> GEMNVDPNNATTTNPSLLLTGVAYSAFNQTSSDACHAAKMLILTSGESKYQVYKWTRGDFDYYSNLRDVTKMSEEAGEGSAYQALAHFFRANYFYQLTLDFGSIPYTDALKAETDANYQPAYDSQEVVLAGILKELEEADKMLEGSDEIISGDIIYNGNLVNWRKLINAYRLRILMSLSGKEKVGDIDVKSEFSKIVADGPLMESLSDNGQLIYLDQQDNRYPYFNDSDFGSGRFMDSTYIAELATRQDPRLFAVATQTPNAEKAGKAINDFSSYDGGDPAVPYSLVNDKAVAGNCSKPAPRYYQTPTNEPMVLLGYVEQQLILAEAVVRGWIQGDDKIYYESAVKASFEFYQKYAVSVA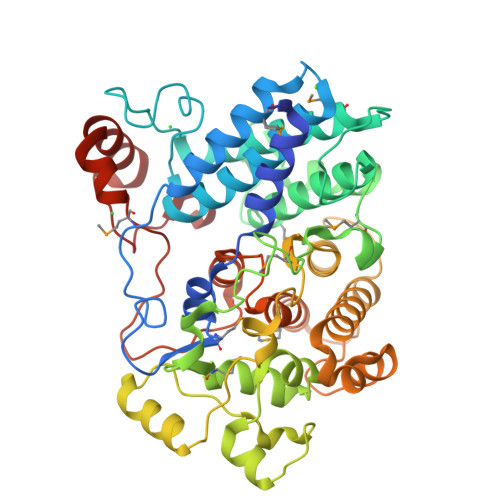DYLTQDAAAEYLRNDKVAYSSSLSTDEKIERIIMQKYLPTFLQGSVWLPYYEALRTGYPDFRRAAGVSLPYRWMYPQDEYNNNATHVEAALNEQFGGSDKTSDKPWWLQ>[4x]KTISFNFNQFHQNEEQLKLQRDARISSNSVLELTKVVNGVPTWNSTGRALYAKPVQVWDS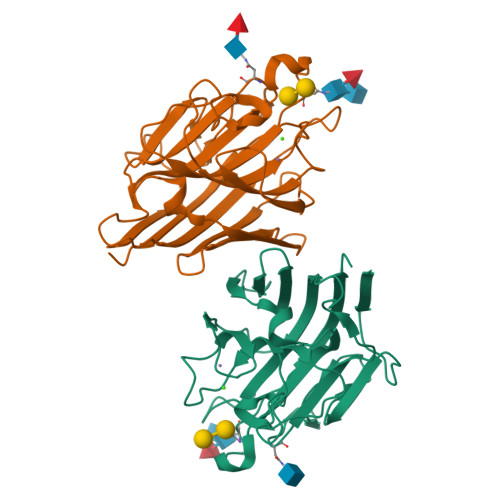TTGNVASFETRFSFSIRQPFPRPHPADGLVFFIAPPNTQTGEGGGYFGIYNPLSPYPFVAVEFDTFRNTWDPQIPHIGIDVNSVISTKTVPFTLDNGGIANVVIKYDASTKILHVVLVFPSLGTIYTIADIVDLKQVLPESVNVGFSAATGDPSGKQRNATETHDILSWSFSASLPGTNEF>MSLILYDYFRSTACYRVRIALNLKKIAYEKIEVHLVNNGGEQHSLQYHQINPQELVPSLDINGQILSQSMAIIDYLEEIHPEMPLLPKDPFMKATLKSMALIVACDMHPLNNLRVLNRLKEQFNANEEQVLEWYHHWLKTGFDAFEEKLGALERDKPVCFGSEVGLADVCLIPQVYNAHRFHFDMASYPIINEINEYCLTLPAFHDAAPEAISSEGHHHHHH[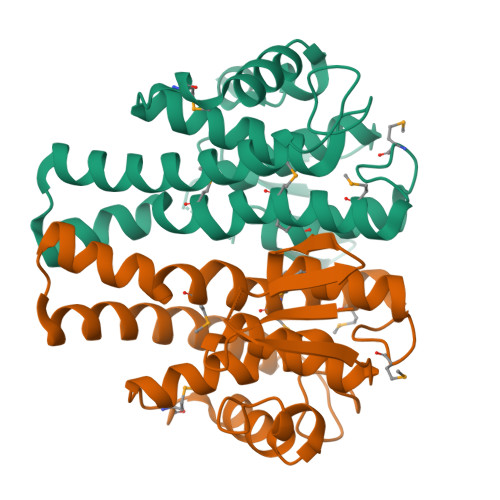4x]>APRKFFVGGNWKMNGDKKSLGELIHTLNGAKLSADTEVVCGAPSIYLDFARQKLDAKIGVAAQNCYKVPKGAFTGEISPAMIKDIGAAWVILGHSERRHVFGESDELIGQKVAHALAEGLGVIACIGEKLDEREAGITEKVVFEQTKAIADNVKDWSKVVLAYEPVWAIGTGKTATPQQAQEVHEKLRGWLKTHVSDAVAQSTRIIYGGSVTGGNCKELASQHDVDGFLVGGASLKPEFVDIIN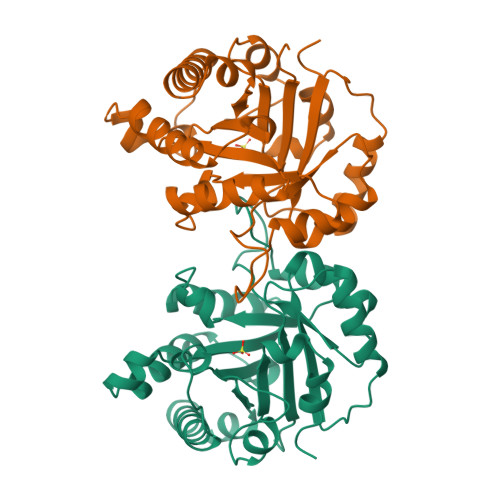AKH[2x]>[8x]MSDFDLYRPTEEHEALREAIRSVAEDKIAPHAADVDEQSRFPQEAYEALRASDFHAPHVAEEYGGVGADALATCIVIEEIARVCASSSLIPAVNKLGSMPLILSGSDEVKQRYLPELASGEAMFSYGLSEREAGSDTASMRTRAVRDGDDWILNGQKSWITNAGISKYYTVMAVTDPDGPRGRNISAFVVHIDDPGFSFGEPERKLGIKGSPTRELIFDNVRIPGDRLVGKVGEGLRTALRTLDHT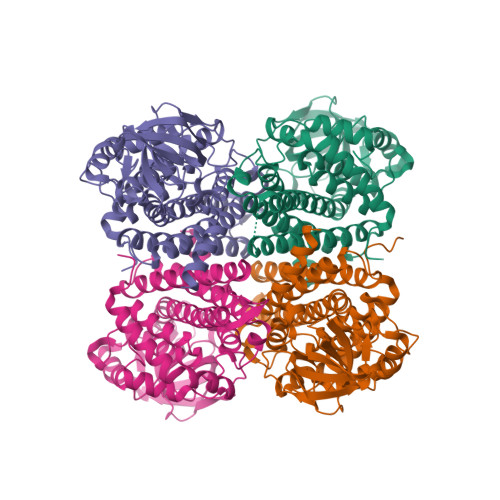RVTIGAQAVGIAQGALDYALGYVKERKQFGKAIADFQGIQFMLADMAMKLEAARQMVYVAAAKSERDDADLSFYGAAAKCFASDVAMEITTDAVQLLGGYGYTRDYPVERMMRDAKITQIYEGTNQIQRVVMARQLLKK Here, we show that the bacterial R28 protein, which is epidemiologically associated with outbreaks of puerperal sepsis, specifically targets the human receptor CEACAM1. This interaction triggers events that would favor the development of puerperal sepsis, including adhesion to cervical cells, suppression of epithelial wound repair and subversion of innate immune responses. The human immunomodulatory receptor CEACAM1 (carcinoembryonic antigen-related cell adhesion molecule 1) binds to some bacterial proteins that contain an Ig-like fold designated IgI3. The IgI3 domain of R28 was sufficient for the interaction, and the N-terminal domain of CEACAM1 was necessary and sufficient for the interaction, as demonstrated in direct binding assays.

We solved the structure of R28-IgI3 bound to CEACAM1-N at a resolution of 3.05 Å. The asymmetric unit contains four copies of the (R28-IgI3)-(CEACAM1-N) complex (the four paired molecules are A-B). The R28 domain has an Ig-like fold belonging to the IgI3 subset, which we recently identified as a domain in the β protein from S. agalactiae that binds CEACAM1 and CEACAM517. Notably, R28-IgI3 has the following properties of the IgI3 fold: A’ and A” strands, lack of C′ and C′′ strands, and a truncated C strand. A notable difference between the structure of the R28-IgI3 domain and the β-IgI3 domain is the presence in R28-IgI3 of a helix-turn-helix (HTH) motif between the C and D strands. We next assessed the mechanism of interaction between R28-IgI3 and CEACAM1-N. In the complex, R28-IgI3 targets the dimerization interface of CEACAM1-N (the A′GFCC′C′′ face) using a pocket of residues (K45, Y61, K64) that have high electrostatic potential. Taken together, our structural and biochemical analysis indicates that R28-IgI3 docks over the CEACAM1 cis/trans dimerization site of the A′GFCC′C′′ face (residues F29, Q89, I91 and L95), and that the unique structural features of R28-IgI3 provide a site with high electrostatic charge (K45 and Y61) and high stability (I52 and I53) for CEACAM1 binding. Mutation of CEACAM1-N at residues F29, I91 or L95 abolished the interaction with R28-IgI3, while mutation of CEACAM1-N at Q89 reduced binding to R28-IgI3. Significant reductions in binding of CEACAM1-N were observed for Dynabeads coated with R28-IgI3 mutated at K45, I52, I53, and Y61. Thus, the analysis indicated that the F29 residue in human CEACAM1 is a critical determinant of human-specificity, likely through interaction with residues K45 and I52 on R28-IgI3.

>[4x]MAQLTTESMPFNVAEGKEVLLLVHNLPQQLFGYSWYKGERVDGNRQIVGYAIGTQQATPGPANSGRETIYPNASLLIQNVTQNDTGFYTLQVIKSDLVNEEATGQFHVY;>TAPTLTVTPEQQTVKVDEDITFTVTVEDENEVELGLDDLKAKYENDIIGARVKIKYLTKEPNKKVMEVTIMKATLADKGAITFTAKDKAGNQAEPKTVTINVLPLKDSNEPKLPSTGGSHHHHHH[4x]> MADTPSSEVIKETKVGSIIQQNNIKYKVLTVEGNIGTVQVGNGVTPVEFEAGQDGKPFTIPTKITVGDKVFTVTEVASQAFSYYPDETGRIVYYPSSITIPSSIKKIQKKGFHGSKAKTIIFDKGSQLEKIEDRAFDFSELEEIELPASLEYIGTSAFSFSQKLKKLTFSSSSKLELISHEAFANLSNLEKLTLPKSVKTLGSNLFRLTTSLKHVDVEEGNESFASVDGVLFSKDKTQLIYYPSQKNDESYKTPKETKELASYSFNKNSYLKKLELNEGLEKIGTFAFADAIKLEEISLPN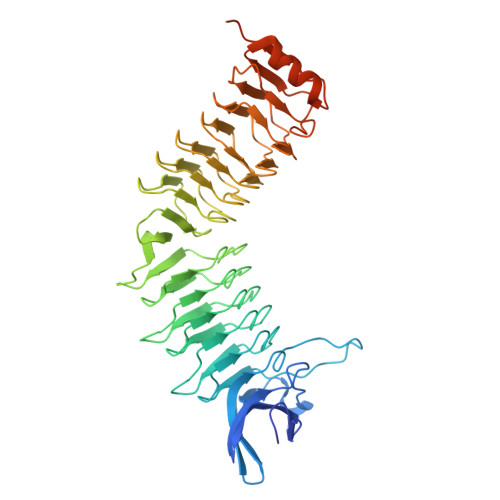SLETIERLAFYGNLELKELILPDNVKNFGKHVMNGLPKLKSLTIGNNINSLPSFFLSGVLDSLKEIHIKNKSTEFSVKKDTFAIPETVKFYVTSEHIKDVLKSNLSTSNDIIVEKVDNIKQETDVAKPKKNSNQGVVGWVKDKG> MNIVLMGLPGAGKGTQADRIVEKYGIPH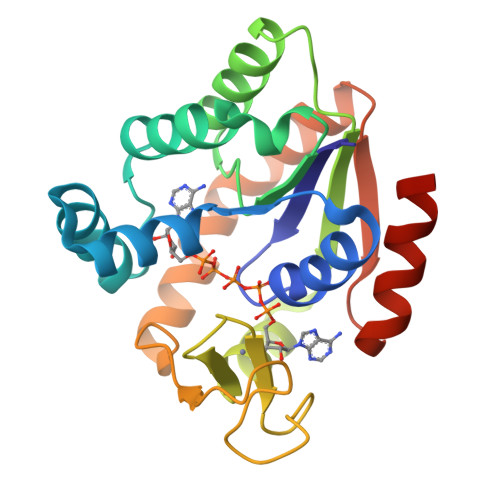ISTGDMFRAAIQEGTELGVKAKSFMDQGALVPDEVTIGIVRERLSKSDCDNGFLLDGFPRTVPQAEALDQLLADMGRKIEHVLNIQVEKEELIARLTGRRICKVCGTSYHLLFNPPQVEGKCDKDGGELYQRADDNPDTVTNRLEVNMNQTAPLLAFYDSKEVLVNINGQKDIKDVFKDLDVILQGNGQ> MSVKLTPDFDNPKWIGRHKHMFNFLDVNHNGRISLDEMVYKASDIVINNLGATPEQAKRHKDAVEAFFGGAGMKYGVETEWPEYIEGWKRLASEELKRYSKNQITLIRLW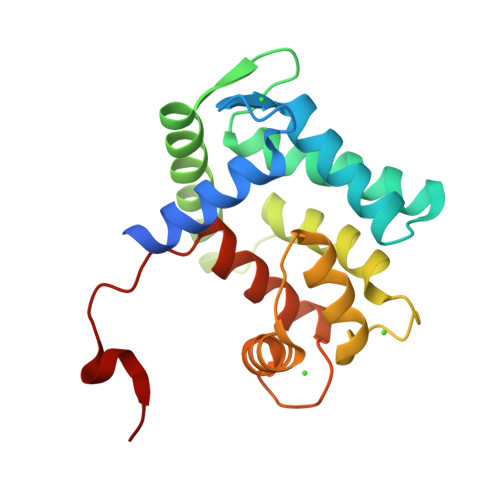GDALFDIIDKDQNGAISLDEWKAYTKSAGIIQSSEDCEETFRVCDIDESGQLDVDEMTRQHLGFWYTMDPACEKLYGGAVP>[4x]GSMQNTTHDNVILELTV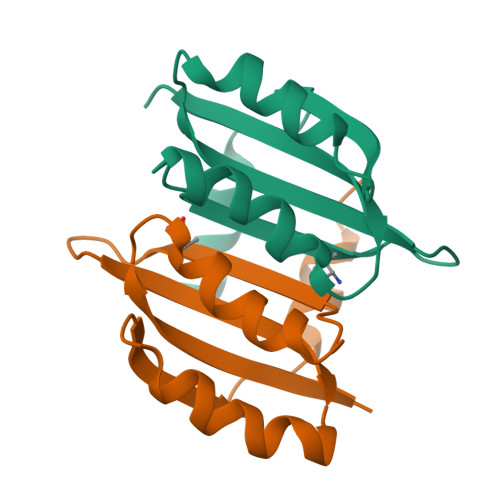RNHPGVMTHVCGLFARRAFNVEGILCLPIQDSDKSHIWLLVNDDQRLEQMISQIDKLEDVVKVQRNQSDPTMFNKIAVFFQ>[3x]GDPNQAVLKFTTEIHPSCVTRQKVIGAGEFGEVYKGMLKTSSGKKEVPVAIKTLKAGYTEKQRVDFLGEAGIMGQFSHHNIIRLEGVISKYKPMMIITEYMENGALDKFLREKDGEFSVLQLVGMLRGIAAGMKYLANMNYVHRDLAARNILVNSNLVCKVSDFGL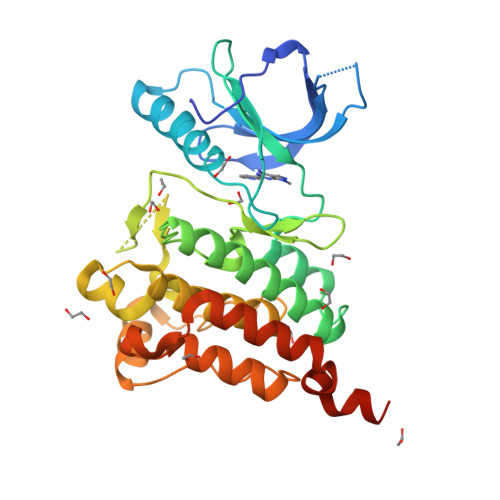SRVLEDDPEATYTTSGGKIPIRWTAPEAISYRKFTSASDVWSFGIVMWEVMTYGERPYWELSNHEVMKAINDGFRLPTPMDCPSAIYQLMMQCWQQERARRPKFADIVSILDKLIRAPDSLKTLADFDPRVSIRLPSTSG>[2x]SNAMNTGEMKINWVSRYMPLLNKIAEEYSREKPLSGFTVGMSIHLEAKTAYLAI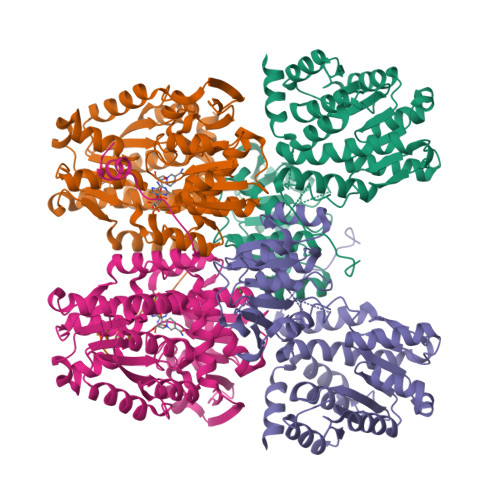TLSKLGAKVVITGSNPLSTQDDVAEALRSKGITVYARRTHDESIYRENLMKVLDERPDFIIDDGGDLTVISHTEREEVLENLKGVSEETTTGVRRLKALEETGKLRVPVIAVNDSKMKYLFDNRYGTGQSTWDAIMRNTNLLVAGKNVVVAGYGWCGRGIALRAAGLGARVIVTEVDPVKAVEAIMDGFTVMPMKEAVKIADFVITASGNTDVLSKEDILSLKDGAVLANAGHFNVEIPVRVLEEIAVEKFEARPNVTGYTLENGKTVFLLAEGRLVNLAAGDGHPVEIMDLSFALQIFAVLYLLENHRKMSPKVYMLPDEIDERVARMKLDSLGVKIDELTEKQRRYLRSWQ>MLEVPTDGNAGLLAEPQIAMFCGRLNMHMNVQNGKWDSDPSGTKTCIDTKEGILQYCQEVYPELQITNVVEANQPVTIQNWCKRGRKQCKTHPHFVIPYRCLVGEFVSDALLVPDKCKFLHQERMDVCETHLHWHTVAKETCSEKSTNLHDYGML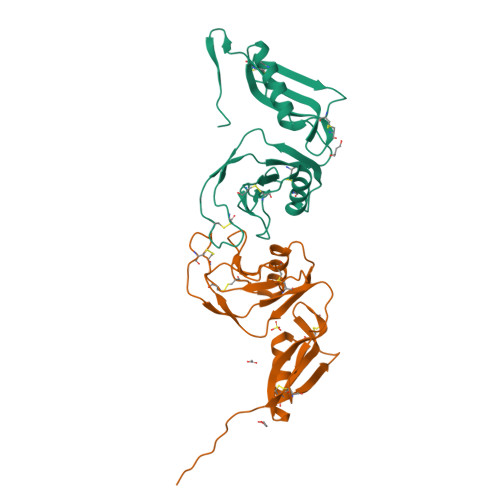LPCGIDKFRGVEFVCCPLAIEGRKLAAALEHHHHHH[8x]>GPDSSLFAPYLPQANIPELIQEGRLVAGILRVNKKNRSDAWVSTDGALDADIYICGSKDRNRALEGDLVAVELLVVDDVWESKKEKEEKKRRKDASMQHDLIPLNSSDDYHNDASVTAATSNNFLSSPSSSDSLSKDDLSVRRKRSSTINNDSDSLSSPTKSGVRRRSSLKQRPTQKKNDDVEVEGQSLLLVEEEEINDKYKPLYAGHVVAVLDRIPGQLFSGTLGLLRPSQQANSDNNKPPQSPKIAWFKPTDKKVPLIAIPTELAPKDFVENADKYSEKLFVASIKRWPITSLHPFGILVSELGDIHDPDTEIDSILRDNNFLSNEYLDQKNPQKEKPSFQPLPLTAESLEYRRNFTDTNEYNIFAISELGWVSEFALHVRNNGNGTLELGCHVVDVTSHIEEGSSVDRRARKRSSAVFMPQKLVNLLPQSFNDELSLAPGKESATLSVVYTLDSSTLRIKSTWVGESTISPSNILSLEQLDEKLSTGSPTSYLSTVQEIARSFYARRINDPEATLLPTLSLLESLDDEKVKVDLNILDRTLGFVVINEIKRKVNSTVAEKIYTKLGDLALLRRQMQPIATKMASFRKKIQNFGYNFDTNTADELIKGVLKIKDDDVRVGIEILLFKTMPRARYFIAGKVDPDQYGHYALNLPIYTHFTAPMRRYADHVVHRQLKAVIHDTPYTEDMEALKITSEYCNFKKDCAYQAQEQAIHLLLCKTINDMGNTTGQLLTMATVLQVYESSFDVFIPEFGIEKRVHGDQLPLIKAEFDGTNRVLELHWQPGVDSATFIPADEKNPKSYRNSIKNKFRSTAAEIANIELDKEAESEPLISDPLSKELSDLHLTVPNLRLPSASDNKQNALEKFISTTETRIENDNYIQEIHELQKIPILLRAEVGMALPCLTVRALNPFMKRV[2x]

Ssd1, a conserved fungal RNA-binding protein, is important in stress responses, cell division and virulence. Ssd1 is closely related to Dis3L2 of the RNase II family of nucleases, but lacks catalytic activity and likely suppresses translation of bound mRNAs. Saccharomyces cerevisiae Ssd1 binds RNA, but does not have detectable exonuclease activity. Transcripts associated with Ssd1 were enriched for mRNAs encoding cell wall biogenesis proteins and Ssd1 was shown to repress their translation.

To better understand the molecular basis for the function of Ssd1 as an RBP, we solved the crystal structure of the core folded domains of Ssd1. This truncated protein lacks the first 338 residues that are predicted to be natively unstructured but is sufficient to bind Ssd1-specific RNA motifs in vitro. Despite the low sequence identity between Ssd1 and yeast Rrp44 or mouse Dis3L2 (22% and 27%, respectively), the structure was solved to 1.9 Å by molecular replacement using fragments of both Rrp44 and Dis3L2. The overall structure of Ssd1 retains the RNB family domain organization: two N-terminal β-barrel cold shock domains (CSD1 and CSD2) sit at the mouth of a funnel-shaped RNB fold. Opposing CSD1 and CSD2 is a C-terminal β-barrel S1 domain. First, active RNase II nucleases have a cluster of four acidic residues that coordinate a divalent cation required for catalysis. These are absent in Ssd1 (5), with the structurally equivalent residues being Ser704, Val709, Glu711 and Phe712; this configuration is unable to coordinate a divalent cation. A similar configuration is observed in Ssd1, representing a second structural change that contributes to loss of activity. This segment blocks the lower tract of the residual active site. We conclude that the S1 insertion locks the autoinhibitory segment in place, ensuring a fixed, inactive conformation. The CSD1 insertion in Ssd1, which is only partially assigned in this structure, folds into an α-helix that blocks the mouth of the funnel, excluding RNA binding at this surface. We conclude that the RNA binding site of Ssd1 is located on the highly conserved outer surface of the cold shock domains and is required for Ssd1 function in vivo.We present crystal structures of a new NAD+-binding riboswitch termed NAD+-II, bound to nicotinamide mononucleotide (NMN), nicotinamide adenine dinucleotide (NAD+) and nicotinamide riboside (NR). The RNA structure comprises a number of structural features including three helices, one of which forms a triple helix by interacting with an A5 strand in its minor-groove, and another formed from a long-range pseudoknot. Unusually the riboswitch binds two molecules of ligand, bound at distinct, non-overlapping sites in the RNA. Binding occurs primarily through the nicotinamide moiety of each ligand, held by specific hydrogen bonding and stacking interactions with the pyridyl ring.

We have determined the structure of the two-strand version of the NAD+-II riboswitch bound to NR at a resolution of 2.87 Å. The RNA structure of the riboswitch bound to NR superimposes very well with that bound to NMN, with an RMSD of 0.365 Å. As with the other complexes, two molecules of NR are observed bound to the RNA, at the same two sites observed for NMN and NAD+. At site 1 the nicotinamide moiety of NR is bound in plane with the G33:C46 base pair, and hydrogen bonded in the same manner. However, because NR lacks the phosphate group there can be no interaction with C5. At site 2 the nicotinamide moiety of NR is bound in plane with the C13:G52 base pair in the major groove of the PK helix, and hydrogen bonded equivalently to that of NMN and NAD+. As with the site 1 because NR lacks the phosphate group there can be no interaction with C10 at the lower end of the PK helix.

> AGAGCGUUGCGUCCGAAAGUCGCC;> GCGACACGGCUCUUUAAAAACAAAAGGAGAA>ASVGADLGLWNRLEPALAYLAPEERAKVREAYRFAEEAHRGQLRRSGEPYITHPVAVAEILAGLQMDADTVAAGLLHDTLEDCGVAPEELERRFGPTVRRIVEGETKVSKLYKLANLEGEERRAEDLRQMFIAMAEDVRIIIVKLADRLHNLRTLEHMPPEKQKRIAQETLEIYAPLAHRLGMGQLKWELEDLSFRYLHPEAFASLSARIQATQEARERLIQKAIHLLQETLARDELLQSQLQGFEVTGRPKHLYSIWKKMEREGKTLEQIYDLLAVRVILDPKPAPTRE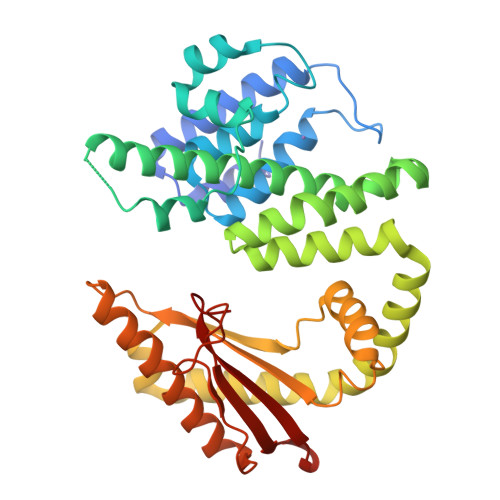SQALREKQVCYHVLGLVHALWQPIPGRVKDYIAVPKPNGYQSLHTTVIALEGLPLEVQIRTREMHR[3x]> MVAITVQGAQLIKRVVERFYPGIAFNINEGACYIYKFSDHIRRIRMKHGTKYRRQAEEIIRNISLRKERLYGIPVLDEVEWKYVFDGQTFQSYAFEVYVNSILPWSELDPEEEFLRNYRVSREMTEVEKFIEFRAKNEMQIYGDIPIKVWCCFINELSAELKHVPLGMQVMADFVNRFDSPFHQGNRDLSNLEDFQVAYTTPLLFEMCCMESILEFNIKMRMREEEISALEFGDMKVDPVGLLREFFILCLPHPKKINNVLRAPYSWFVKMWGVGADPIVVLQSTAGDDRNSKDVFYDKFRTEPNRYKALFRSSFYNESRRMNEEKILEAVKYSQKLGSHDRRLPLFEKMLKTVYTTPFYPHKSSNMILASFLLSIQTITGYGRAWVKNVSTEFDKQLKPNPSNLVQDVSDLTREFFKQAYVEAKERREEIVKPEDLYTSMLRLARNTSSGFSTEIYVKKRFGPRLRDKDLIKINSRIKALVIFTKGHTVFTDEELHKKYNSVELYQTKGSRDVPIKATRTIYSINLSVLVPQLIVTLPLNEYFSRVGGITSPDYKKIGGKVIVGDLEATGSRVMDAADCFRNSADRDIFTIAIDYSEYDTHLTRHNFRTGMLQGIREAMAPYRDLRYEGYTLEQIIDFGYGEGRVANTLWNGKRRLFKTTFDAYIRLDESERDKGSFKVPKGVLPVSSVDVANRIAVDKGFDTLIAATDGSDLALIDTHLSGENSTLIANSMHNMAIGTLMQREVGREQPGVLTFLSEQYVGDDTLFYTKLHTTDTKVFDKVAASIFDTVAKCGHEASPSKTMMTPYSVEKTQTHAKQGCYVPQDRMMIISSERRKDIEDVQGYVRSQVQTMITKVSRGFCHDLAQLILMLKTTFIGAWKMKRTIKEDAMYRDRKFDSNDEDGFTLIQIRNPLALYVPIGWNGYGAHPAALNIVMTEEMYVDSIMISKLDEIMAPIRRIVHDIPPCWNETQGDKRGLISATKMSFFSKMARPAVQAALSDPQIINLVEELPLGEFSPGRISRTMMHSALLKESSARTLLSSGYELEYQKALNSWITQVSMRLGEESGVISTSYAKLFDVYFEGEL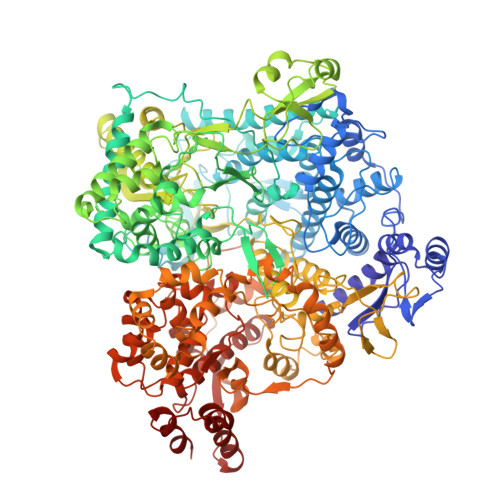DGAPHMFPDQNLSPQFYIQKMMIGPRVSSRVRNSYVDRIDVILRKDVVMRGFITANTILNVIEKLGTNHSVGDLVTVFTLMNIETRVAEELAEYMTSEKIRFDALKLLKKGIAGDEFTMSLNVATQDFIDTYLAYPYQLTKTEVDAISLYCTQMIMLRAALGLPKKKMKIVVTDDAKKRYKIRLQRFRTHVPKIKVLKKLIDPNRMTVRNLENQFV> MSATKSIVGEALEYVNIGLSHFLALPLAQRISLIIIIPFIYNIVWQLLYSLRKDRPPLVFYWIPWVGSAVVYEMKPYEFFEECQKKYGDIFSFVLLGRVMTVYLGPKGHEFVFNAKLADVSAEAAYAHLTTPVFGKGVIYDCPNSRLMEQKKFVKGALTKEAFKSYVPLIAEEVYKYFRDSKNFRLNERTTGTIDVMVTQPEMTIFTASRSLLGKEMRAKLDTDFAYLYSDLDKGFTPINFVFPNLPLEHYRKRDHAQKAISGTYMSLIKERRKNNDIQDRDLIDSLMKNSTYKDGVKMTDQEIANLLIGVLMGGQHTSAATSAWILLHLAERPDVQQELYEEQMRVLDGGKKELTYDLLQEMPLLNQTIKETLRMHHPLHSLFRKVMKDMHVPNTSYVIPAGYHVLVSPGYTHLRDEYFPNAHQFNIHRWNNDSASSYSVGEEVDYGFGAISKGVSSPYLPFGGGRHRCIGEHFAYCQLGVLMSIF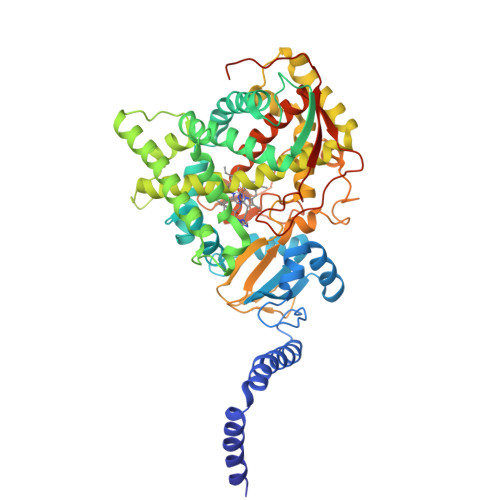IRTLKWHYPEGKTVPPPDFTSMVTLPTGPAKIIWEKRNPEQKIGGRHHHHHH> REFTIDFSTQQSYVSSLNSIRTEISTPLEHISQGTTSVSVINHTPPGSYFAVDIRGLDVYQARFDHLRLIIEQNNLYVAGFVNTATNTFYRFSDFTHISVPGVTTVSMTTDSSYTTLQRVAALERSGMQISRHSLVSSYLALMEFSGNTMTRDASRAVLRFVTVTAEALRFRQIQREFRQALSETAPVYTMTPGDVDLTLNWGRISNVLPEYRGEDGVRVGRISFNNISAILGTVAVILNCHHQGARSVRAVNEESQPECQITGDRPVIKINNTLWESNTAAAFLNRKSQFLYTTGK;>[5x]ADCAKGKIEFSKYNEDDTFTVKVDGKEYWTSRWNLQPLLQSAQLTGMTVTIKSSTCESGSGFAEVQFNND

Shiga toxin (Stx), a major virulence factor of enterohemorrhagic Escherichia coli (EHEC), can cause fatal systemic complications. All Stx proteins consist of a catalytic A-subunit and a B-subunit pentamer. The catalytic A-subunit, which is a member of ribosome-inactivating proteins (RIPs), has an RNA N-glycosidase activity that cleaves a specific adenine from 28S ribosomal RNA to inhibit eukaryotic protein synthesis. The B-subunit pentamer functions to bind Galα[1–4]–Galβ[1–4]–Glcβ-ceramide (Gb3), a glycolipid present on the surface of target cells.

To elucidate the precise manner by which these shorter peptides bind to Stx2a, X-ray crystallography analysis was performed with co-crystals of each peptide and the Stx2a holotoxin, which were obtained via the soaking method. We were able to determine electron densities for AR4A-mono, R4A-mono, R3A-mono, and R2A-mono, and X-ray crystal structures were solved to final resolutions of 1.80, 1.80, 1.90, and 1.75 Å-resolution, respectively. These structures reveal that the AR4A-mono, R4A-mono, R3A-mono, and R2A-mono peptides bind tightly to the catalytic A-subunit. In all cases, the common Arg8-Arg9-Ala10 motif (numbering reflects residue position in full-length MMβA-mono) interacts equally with the Glu72, Tyr77, Val78, Asp94, Ser112, Tyr114, Thr115, Glu167, Arg170, Thr199, and Gly203 residues present in the catalytic pocket of the A-subunit, whereas the Arg8 and Arg9 residues of the motif electrostatically interact with Glu167 and Asp94, respectively. The amide group of the Ala10, but not its side chain, interacts with the Val78, Ser112 and Arg170 residues. Overall, we find that the binding patterns of these shorter peptides are almost identical to that of MMβA-mono. Combined with results from the competition assay, these data demonstrate that these shorter peptides efficiently bind to the A-subunit of Stx2a, and R2A-mono is the minimal essential motif needed for binding. Using X-ray crystal structural analysis, we clearly show direct binding between R2A-mono and the A-subunit, in a manner that is identical to that of the Arg8-Arg9-Ala10 region of full-length MMβA-mono. We found that R4-mono, AR4A-mono, R4A-mono, and R3-mono exhibit greater inhibitory effects (relative IC50 values = 0.387, 2.27, 2.70, and 3.68 µM, respectively) than non-tagged MMβA-mono (relative IC50 = 8.14 µM), which was used as a positive control to compete the binding. Notably, R3A-mono and R2A-mono (relative IC50 values = 89.6 and 132 µM, respectively) also substantially inhibit binding, albeit with efficacies less than that of MMβA-mono. All peptides, including R2A-mono, were found to efficiently inhibit Stx2a toxicity, confirming that R2A-mono, which is a minimal essential motif for binding, is sufficient for effective inhibition of Stx2a.>[4x]MDVDLGKLFFCGFDDFNEEAREVIQKYRPAGVLIYPGVLSKEYLF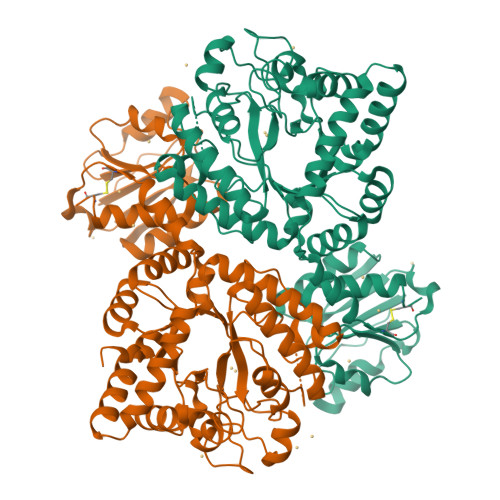LDFMNFLSRNGRFIVSSDHEGGQLEVLKYVPSFPGNLAAGKVDPVFTGRYCEMAGRIMNTLGFNMVFAPVLDLLSEKGSAVVDLRSFGSDPEVVASHGMEACMGYFKGGVIPCIKHFPGHGKTADDSHYLLPTVNASFEELWREDLLPFRRIFQSRVKTAVMTAHVKYPAVDDLPATLSKKLITEVLREKLNFKGLVLSDAMEMKAISENFSVEEAVRFFIEAGGNMILLDNFRDLPVYYESLKKLIEDGSIERGKVERSIKIVDEYLSALENRFNSGLIAEVAERAIECTRMRKELLGREVVLLVPSNKNLSPADTTGDDYDLIPEVAKRFFKVRDVIRYDIEAGPDDVDGELIFDFVVNASKNEQVLQAHLSLPSDRTIYFIIRNPFDAKFFPGRSVVITHSTKPISVYKSFQHLLGRCS>SMKLDIKKTFSNRSDRVKGIDFHPTEPWVLTTLASGRVEIWNYETQVEVRSIQVTETPVRAGKF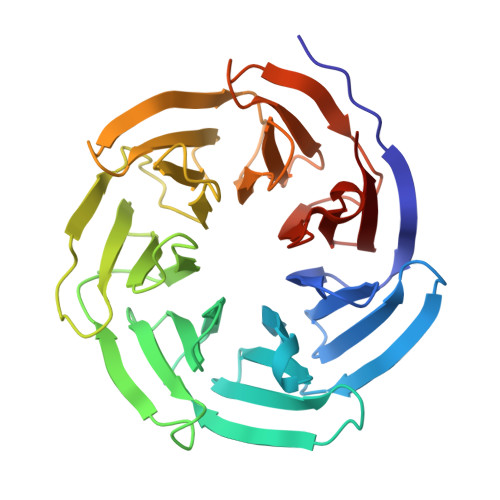IARKNWIIVGSDDFRIRVFNYNTGEKVVDFEAHPDYIRSIAVHPTKPYVLSGSDDLTVKLWNWENNWALEQTFEGHEHFVMCVAFNPKDPSTFASGCLDRTVKVWSLGQSTPNFTLTTGQERGVNYVDYYPLPDKPYMITASDDLTIKIWDYQTKSCVATLEGHMSNVSFAVFHPTLPIIISGSEDGTLKIWNSSTYKVEKTLNVGLERSWCIATHPTGRKNYIASGFDNGFTVLSLG[2x];> GVKLHYE> CDIHVLWEWKCFEEL;>EVVKFMDVYQRSYCHPIETLVDIFQEYPDEIEYIFKPSCVPLMRCGGCCNDEGLECVPTEESNITMQIMRIKPHQGQHIGE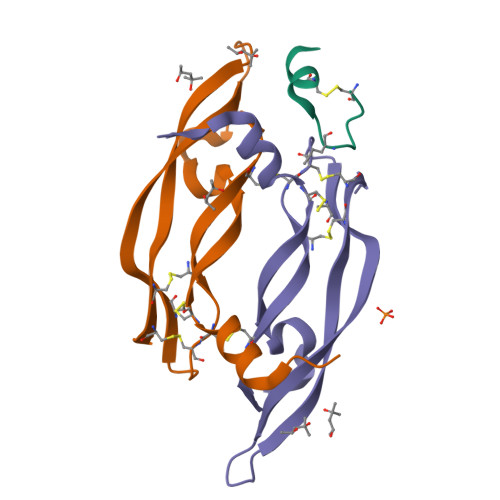MSFLQHNKCECRPK[2x]>MSSDADAHKVGLIPVTLMVSGNIMGSGVFLLPANLASTGGIAIYGWLVTIIGALGLSMVYAKMSFLDPSPGGSYAYARRCFGPFLGYQTNVLYWLACWIGNIAMVVIGVGYLSYFFPILKDPLVLTITCVVVLWIFVLLNIVGPKMITRVQAVATVLALIPIVGIAVFGWFWFRGETYMAAWNVSGLGTFGAIQSTLNVTLWSFIGVESASVAAGVVKNPKRNVPIATIGGVLIAAVCYVLSTTAIMGMIPNAALRVSASPFGDAARMALGDTAGAIVSFCAAAGCLGSLGGWTLLAGQTAKAAADDGLFPPIFARVNKAGTPVAGLIIVGILMTIFQLSSISPNATKEFGLVSSVSVIFTLVPYLYTCAALLLLGHGHFGKARPAYLAVTTIAFLYCIWAVVGSGAKEVMWSFVTLMVITAMYALNYNRLHKNPYPLDAPISKDLELEVLFQ[2x]

The membrane transport protein AdiC is part of the arginine-dependent acid resistance system of Escherichia coli. The L-arginine/agmatine transporter AdiC belongs to the amino acid/polyamine/organocation (APC) transporter superfamily and is a prokaryotic member of the SLC7 family of solute carriers. AdiC forms a homodimer in detergent micelles and lipid membranes, and each monomer is a self-contained transporter. Functional studies have shown that AdiC is an obligate exchanger, coupling influx of L-arginine with efflux of agmatine across the lipid bilayer.

In this study, we present the structure of the L-arginine/agmatine transporter AdiC in the outward-open substrate-free state at the unprecedented resolution of 1.7 Å. AdiC is homodimeric and each monomer consists of twelve transmembrane α-helices (TMs) with intracellular N- and C-termini. The significant increase in resolution in the presented high-resolution structure, allowed us to identify twenty-one and fifteen water molecules in monomers A and B, respectively. In summary, we suggest that binding of L-arginine to AdiC in the outward-open conformation replaces water molecules H2O3, H2O5, H2O6, H2O7, H2O13, H2O17, and H2O19. The side chain of W202 (TM6a) in the outward-open conformation forms hydrogen bonds with two water molecules: H2Oα and H2Oβ. However, in the molecular dynamics (MD) simulations, the observed water network (H2Oα-H2Oγ) interacting with W202 in the AdiC crystal structure was disrupted, allowing W202 to sample a large range of conformations. In contrast to W202, the spatial orientation of W293 is stabilized by a hydrogen bond to H2O9. We identified a heart-shaped cavity at the interface of the AdiC dimer that is lined by mostly hydrophobic amino acids, F84, L85, V363, L366, F414, L417, and M418, and a few polar groups, Q88, Y367, and T421. Therefore, we hypothesized the presence of a dynamic interfacial water network and placed water molecules into these Fo-Fc densities during refinement. This resulted in the identification of eleven water molecules in the interdimeric cavity. In all cases, the thermostability of AdiC was significantly reduced, supporting the importance of water for dimer stabilization.> MERYENLFAQLNDRREGAFVPFVTLGDPGIEQSLKIIDTLIDAGADALELGVPFSDPLANGPTIQNANLRAFAAGVTPAQCFEMLALIREKHPTIPIGLLMYANLVFNNGIDAFYARCEQVGVDSVLVADVPVEESAPFRQAALRHNIAPIFICPPNADDDLLRQVASYGRGYTYLLSRSGVTGAENRGALPLHHLIEKLKEYHAAPALQGFGISSPEQVSAAVRAGAAGAISGSAIVKIIEKNLASPK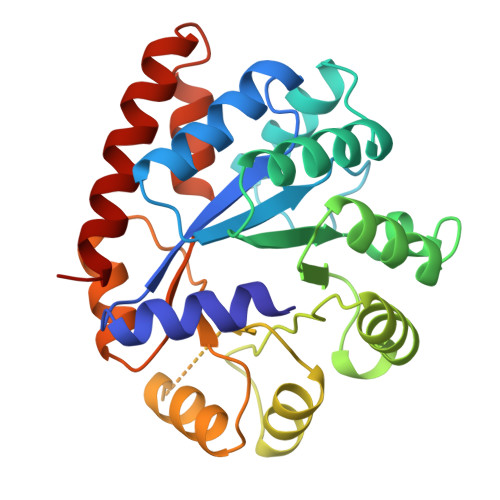QMLAELRSFVSAMKAASRA> 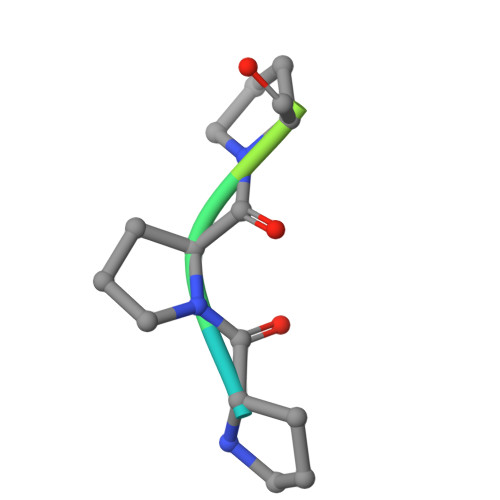LPPPFGPGM The Mononegavirales order groups five families of monopartite, negative-strand RNA viruses many of which are highly pathogenic and/or contagious; the Filoviridae (of which Ebola virus is a representative), the Bornaviridae (Borna disease virus), the Nyamiviridae (midway virus), the Rhabdoviridae (rabies, vesicular stomatitis virus (VSV)) and the Paramyxoviridae (measles virus, human metapneumovirus (hMPV)). These viruses encode a large RNA polymerase (L) (usually >2,000 amino acids) that is crucial to viral replication. As a part of this study, we expressed CR-VI+, a 406-residue fragment comprising CR-VI and the adjoining ‘+ domain’, the variable region carrying the K-K-G-motif, investigated its MTase activity and solved its crystal structure. Besides sequentially methylating the 2′O and N7 atoms of small capped RNAs, CR-VI+ also 2′O methylates uncapped substrates and displays nucleotide triphosphatase (NTPase) activity. Both the CR-VI domain, which assumes a fairly standard MTase fold, and the K-K-G motif of the (mainly helical) +domain are required for the MTase reactions.

Most notably, hMPV and flaviviruses share an unusually long (∼10 residues), flexible β2λ (that is, the loop immediately following the β2-strand), which forms the SAM-binding pocket (SAMP) along with loops β1λ and β4λ, shielding it from the solvent. In CR-VI+, β2λ similarly assumes alternate conformations. Loops β1λ and β4λ also show a degree of flexibility. β1λ residue E1697, conserved in paramyxo- and filoviruses, forms a hydrogen bond with the NH2 group of SAM and is essential for both MTase activities. However, in the absence of SAM, its side chain either moves into the sub-pocket that normally accommodates the NH2 group, or, more markedly, turns towards the solvent in the direction of β2λ, which in this case assumes the ‘open’ position. β4λ forms a side wall of SAMP, and together with αD and β5 also defines a deep, hydrophobic cavity not present in other MTases, termed NSP (or nucleoside-binding pocket).

>[2x]MALLTPIPSPMVNLTQVIDPTEQLAYFPKITFERLKNYDTSSNYAKGKLTRNYMILLPWQHVNRYNFVFSSTGCKVSLKTCIGKLMKDLNPKVLYFIGEGAGNWMARTACEYPDIKFVYRSLKDDLDHHYPLEYQRVIGELSRIIDSGEGLSMETTDATQKTHWDLIHRVSKDALLITLCDAEFKDRDDFFKMVILWRKHVLSCRICTTYGTDLYLFAKYHAKDCNVKLPFFVRSVATFIMQGSKLSGSECYILLTLGHHNNLPCHGEIQNSKMKIAVCNDFYAAKKLDNKSIEANCKSLLSGLRIPINKKELNRQRRLLTLQSNHSSVATVGGSKVIESKWLTNKANTIIDWLEHILNSPKGELNYDFFEALENTYPNMIKLIDNLGNAEIKKLIKVTGYMLVSKKSGHHHHHH>[8x]MGHHHHHHVSSTNGFSATRSTVIQLLNNISTKREVEQYLKYFTSVSQQQFAVIKVGGAIISDNLHELASCLAFLYHVGLYPIVLHGTGPQVNGRLEAQGIEPDYIDGIRITDEHTMAVVRKCFLEQNLKLVTALEQLGVRARPITSGVFTADYLDKDKYKLVGNIKSVTKEPIEASIKAGALPILTSLAETASGQMLNVNADVAAGELARVFEPLKIVYLNEKGGIINGSTGEKISMINLDEEYDDLMKQSWVKYGTKLKIREIKELLDYLPRSSSVAIINVQDLQKELFTDSGAGTMIRRGYKLVKRSSIGEFPSADALRKALQRDAGISSGKESVASYLRYLENSDFVSYADEPLEAVAIVKKDTNVPTLDKFVCSDAAWLNNVTDNVFNVLRRDFPALQWVVSENDANIAWHFDKSQGSYLKGGKVLFWYGIDDINTISELVENFVKSCDTASTLNSSASS

The first step of the route is the production of N-acetyl-L-glutamate (NAG), while the second is the phosphorylation of NAG by NAG kinase (NAGK). We report here structural and functional studies on the arginine-sensitive NAGK from Saccharomyces cerevisiae (yNAGK). The structure of the mature yNAGK, lacking the N-terminal mitochondrial targeting sequence (residues 1–57), reveals an unexpected novel tetrameric architecture, which can be described as a dimer of dimers with D2 symmetry. The AAK domains occupy the center of the molecule flanked by two pairs of interacting DUF619 domains.

The full-length enzyme tetramers consist of the AAK domains occupying the central part of the molecule, as in the truncated enzyme structure, flanked at both ends along the Q axis by a pair of interacting DUF619 domains. The lines joining the centers of mass of mutually interacting DUF619 domains are oblique in relation to the flat AAK tetramer; thus DUF619 domain pairs protrude from the plane defined by the four AAK domains. The structures of the four tetramers found in the two crystals deviate from perfect D2 molecular symmetry, with three subunits in each tetramer exhibiting the open AAK domain conformation. The degree of AAK domain opening is even higher than in the arginine-containing subunit of the truncated enzyme, corresponding to a 20° rotation of the C-lobe. The pulling of the C-lobes by the paired DUF619 domains possibly contributes to this opening of the AAK domain, which is associated with rotations of up to 55° of the DUF619 domain around a hinge located at the AAK domain-DUF619 domain linker (351GYK). The DUF619 domain is a bilobar (N-moiety, residues 354–447; C-moiety, residues 448–502) open αβα sandwich nucleated by a 7-stranded antiparallel β-sheet, which has the characteristic architecture of the histone acetyltransferase fold (GNAT fold). The comparison of the GNAT domains from NgNAGS and yNAGK (with an r.m.s.d. of 2.52 Å for 111 residues) explains why yNAGK lacks NAGS activity. The AcCoA binding site in NgNAGS, found on the boundary of the N- and C-moieties, is blocked in yNAGK (compare Figures 8E and 8F). W431, sandwiched between N460 and T436, blocks the part of the site where the pyrophosphate moiety of the CoA molecule would be expected to bind, thus rendering impossible AcCoA binding. The pairing of the DUF619 domains on each side of the yNAGK tetramer involves hydrophobic interactions between the E′ and F′ helices as well as the continuity of the central β sheets by way of antiparallel bonding of strands 6′ from both domains. These interactions are maintained in the four pairs of DUF619 domains observed in the present crystal structure (with r.m.s.d.s from 0.85 to 1.45 Å), despite the important departures from the D2 symmetry observed in the yNAGK tetramers.6-chloranyl-~{N}-(cyclopropylmethyl)-3-(2~{H}-indazol-5-yl)imidazo[1,2-b]pyridazin-8-amine 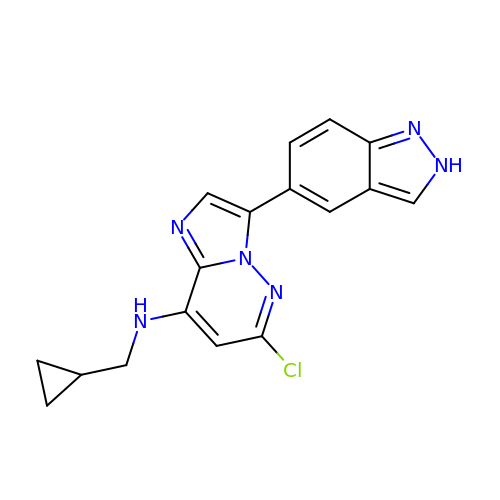| C17 H15 Cl N6 | FLFMYUGDCXTOQI-UHFFFAOYSA-N>[2x]STRATKRQRDQLRQCFDARLTDVAANAAAQAWQDEYEAAVEPLRQAMLGVLAEVAAVRDAAGGQPATASGLSQALSNARIRFFKRFAALHGQR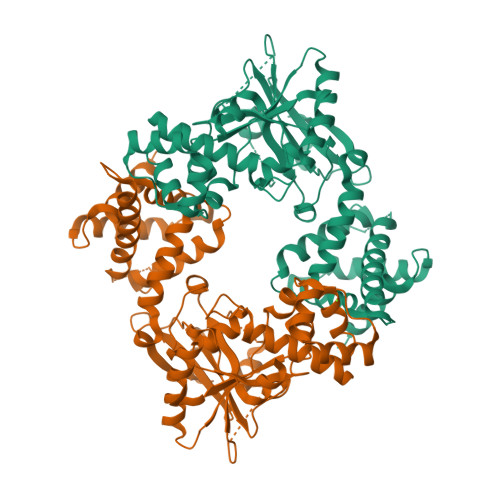GNSACGLHFLIQLRADMLRWHKRIPGLRELDEDLEALFSNWFDVGLLELQPITWDSPASLLEKLIRYEAVHEISSWTDLRNRLDSDRRCYAFFHPRIPREPLIFVEVAFVPEMAANVQALLDEAAPLEDLRRVKWAIFYSISNTQAGLRGVSFGNFLLKRVIEELQREHPKLKQFATLSPIPGFADWLRKRDGESIDRVLGVKRLARWREQHGEVPADGAAWFSALSADTEDTVIRDTAMTLAAHYLVREGGKGVPADPVARFHLGNGACVERVNWGADMSRKGRAQSCGMMVNYLYVPDALDDNLARLGDGNPRISRAVAKLLAAALEHHHHHH>[4x]SQGRACLSKAELTADLIWLSANRTGEESAEELNYSGCDLSGLSLVGLNLSSVNFSGAVLDDTDLRMSDLSQAVLENCSFKNSILNECNFCYANLSNCIIRALFENSNFSNSNLKNASFKGSSYIQYPPILNEADLTGAIIIPGMVLSGAILGDVKELFSEKSNTINLGGCYIDLSDIQENILSVLDNYTKSNKSILLTMNTSDDKYNHDKVR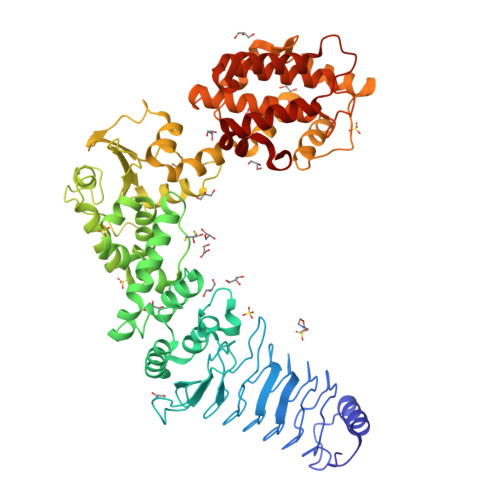AAEELIKKISLDELAAFRPYVKMSLADSFSIHPYLNNANIQQWLEPICDDFFDTIMSWFNNSIMMYMENGSLLQAGMYFERHPGAMVSYNSSFIQIVMNGSRRDGMQERFRELYEVYLKNEKVYPVTQQSDFGLCDGSGKPDWDDDSDLAYNWVLLSSQDDGMAMMCSLSHMVDMLSPNTSTNWMSFFLYKDGEVQNTFGYSLSNLFSESFPIFSIPYHKAFSQNFVSGILDILISDNELKERFIEALNSNKSDYKMIADDQQRKLACVWNPFLDGWELNAQHVDMIMGSHVLKDMPLRKQAEILFCLGGVFCKYSSSDMFGTEYDSPEILRRYANGLIEQAYKTDPQVFGSVYYYNDILDRLQGRNNVFTCTAVLTDMLTEHAKESFPEIFSLYYPVAWR>MHHHHHHSSGRENLYFQGERNYNKWAESYIKYNLSNLKIEKEDLTIYFDNLQVSGNACVSIRKGKQINSFEYIIKFEWLYSKKKEGKDYFGGSVEIPDFSTFSLEENDYAINIERTDESENLRFIYDSILKKEGKEKIK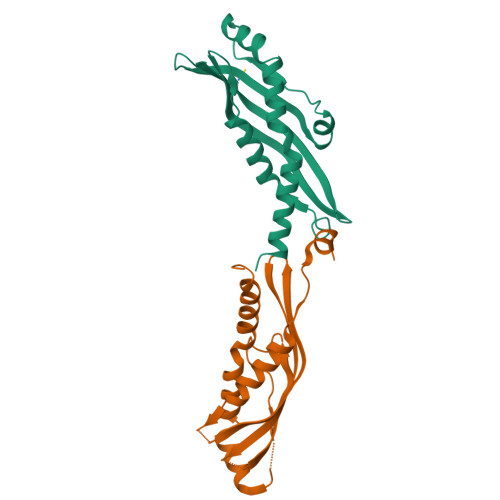ECLKNFQEDLLKHDKNESNKELKIK[2x]> 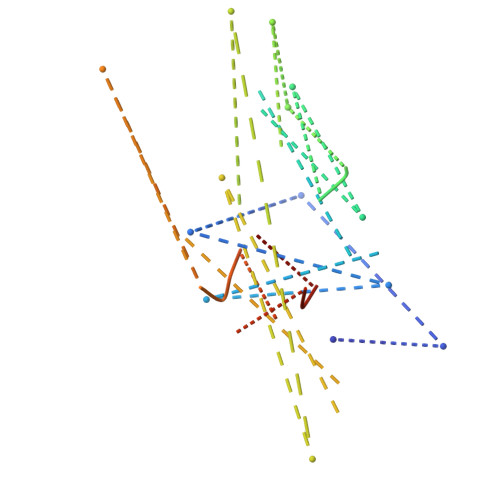SISDYTEAEFVQLLKEIEKENVAATDDVLDVLLEHFVKIT> MHEWALA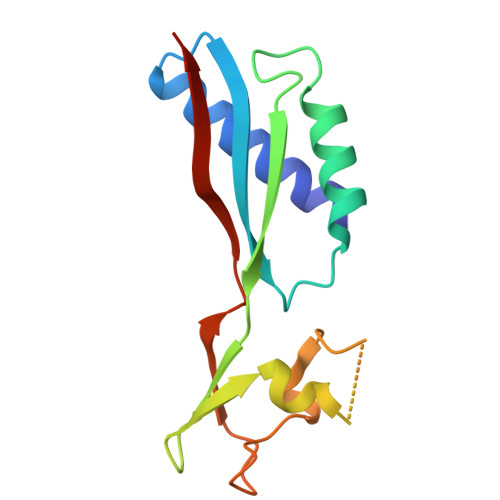DAIVRTVLDYAQREGASRVKAVRVVLGELQDVAEDIVKFAMEQLFAGTIAEGAEIEFVEEEAVFKCRNCNYEWKLKEVKDKFDERIKEDIHFIPEVVHAFLACPKCGSHDFEVVKGRGVYVAGIKIEKEGGS> MVSKRKLSKIDAAEESSKTDLQSRCPETKRSRISDKRAPSQGGLENEGVFEELLRTSGIILKVGEGQNEIAVDQTAFQKKLRVALEKHPSYPGVVNEFISGLESHIKDRSQFKNCLLPCTPARTEGSRTLVHSYCESLIKLLLGIKILQPAVVTLLLEKIPEFFFDVVGTFGTNFPRLIVNQFKWLDGLLDSQDLVKKLMQMLSVSPVPIQHDIITSLPEILEDSQQNEVARELSCLLKQGRRLTVPILDALSRLDLDAELLAKVRQSAMTIVPSVKLEDLPVVIKFILHNVKAADAVEVISDLRKSLDLSSCVLPLQLLGSQRKLKSQAQASSSMSQVTTSQNCVKLLFDVIKLAVRFQKDVSEAWIKAIENSTSVSDHKVLDLIVLLLIHSTNSKNRKQTEKVLRSKIRLGCMPEQLMQNAFQNHSMVIKDFFPSILSLAQTFLHSAHPAVVSFGSCMYKQAFAVFDSYCQQEVVCALVTHVCSGNETELDISLDVLTDLVILHPSLLLRYATFVKTILDSMQKLNPCQIRKLFYILSTLAFSQRQEGSYIQDDMHMVIRKWLSSSVPNHKQMGIIGAVTMMGSVALKRNEADGGLLERPELSIECDGQLSTLLDLVGFCCEQTPEVLALYYDELANLIEKQKGNLDLQLLDKFGKSLVEDFPNDFVVDLSPTVDGSFLFPVKSLYNLDEDETQGAIAINLLPLVSQSEPGRVADEMSNSRKRVVSPICLSPCFRLLRLYTGEQNNGSLEEIDALLGCPLYLTDLEVEGKLDSLSKQEREFLCSLLFYALNWFREVVNAFCQQQDAEMKGKVLTRLQNITELQNVLGKCLAATPGYVPPPATFDSEAPEGVPSINAGGPVRKKNGKKRKSDSSKACSAERTQADESSDGNQPDTELSELEKSAAEKETGNPLAQLQSYRPYFRELDLEVFSVLHCGLLTKSILDTEMHTEASEVVQLGPAELCFLLDDMCWKLEHVLTPGSTRRVPFLKERGNKDVGFSHLCQRSPKEVAVCVVKLLKPLCNHMENMHNYFQTVIPNQGVVDESGLNIQEYQLMSSCYHQLLLAFRLLFAWSGFSQHENSNLLRSALQVLADRLKPGETEFLPLEELISESFQYLLNFQASIPSFQCAFILTQVLMAISEKPMTGWKREKMASLAKQFLCQSWMKPGGDREKGSHFNSALHTLLCVYLEHTDNILKAIEEISSVGVPELINSAKDGCSSTYPTLSRQTFPVFFRVMMAQLESSVKSIPAGKPSDSGEVQLEKLLKWNIAVRNFHILINLVKVFDSRPVLSICLKYGRLFVEAFLKLAMPLLDHSFKKHRDDVQSLLKTLQLSTRQLHHMCGHSKIHQDLGLTNHVPLLKKSLEQFVYRVKAMLAFNHCQEAFWVGVLKNRDLQGEEILSQASAAPEEDSAEGSEEDTEDSAAEEPDGTDSDSGGAGR;> MAQRILQLAAEGSPERLQEALQGLTEGELGDMVTRQALRGRETAALLKGIFKGSPCSQQSGVLRRLQVYKHCVSLVESGDLHVGKVSEIIGLLMLEARQLPGHALAELATLFVEVIKRGSLSNGKSLELFSTVLTALSNSKESLAYGKGELNGEEFKKQLINTLCSSKWDPQCVIHLANMFRDIPLSGEELQFVVEKVLRMFSKLDLQEIPPLVYQLLLLSAKGSKKTVLEGIISFFNQLDKRQKEEQRVPQSADLEVATVPLDQLRHVEGTVILHIVSAINLDQDIGEELIKHLKTEQQKDPGKALCPFSVSLLLSTAVKHRLQEQIFDFLKTSITRSCKDLQILQASKFLQDLCPQQYDVTAVILEVVKNSAFGWDHVTQGLVDLGFSLMESYEPKKSFGGKAAETNLGLSKMPAQQACKLGASILLETFKVHEPIRSDILEQVLNRVLTKAASPVSHFIDLLSNIVVSAPLVLQNSSSRVTETFDNLSFLPIDTVQGLLRAVQPLLKVSMSVRDSLILVLQKAIFSRQLDARKAAVAGFLLLLRNFKILGSLTSSQCSQAIGATQVQADVHACYNSAANEAFCLEILGSLRRCLSQQADVRLMLYEGFYDVLRRNSQLASSIMETLLSQIKQYYLPQQDLLPPLKLEGCIMAQGDQIFLQEPLAHLLCCIQHCLAWYKSTVHLCKGAEDEEEEEDVGFEQNFEEMLESVTRRMIKSELEDFELDKSADFSPSSGVGVKNNIYAIQVMGICEVLIEYNFKIGNFSKNKFEDVLGLFTCYNKLSEILKEKAGKNKSTLGNRIARSFLSMGFVSTLLTALFRDNAQSHEESLAVLRSSTEFMRYAVSVALQKVQQLEEMGQTDGPDGQNPEKMFQNLCKITRVLLWRYTSIPTAVEESGKKKGKSISLLCLEGLLRIFNTMQQLYAARIPQFLQALDITDGDAEEADINVTEKAAFQIRQFQRSLVNQLSSAEDDFNSKETQLLITILSTLSKLLDPGSQQFLQFLTWTVKICKENALEDLSCCKGLLTLLFSLHVLYKSPVSLLRELAQDIHACLGDIDQDVEIESRSHFAIVNVKTAAPTVCLLVLGQADKVLEEVDWLIKRLTILGSDTSEDSTQASNQTQALEKGVILQLGTLLTVFHELVQTALPAGSCVDSLLRSLSKTYAILTSLIKHYIQACRSTSNTVPGRLEKLVKLSGSHLTPQCYSFI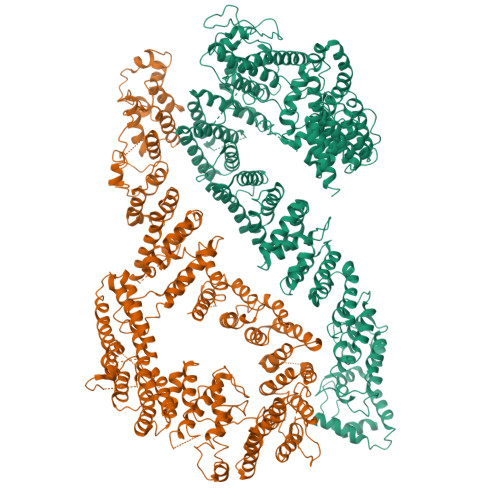TYVQNIHSESLSFAEEKKKKKKEDETAVVSTVMAKVLRDTKPIPNLIFAIEQYEKFLIHLSKKSKVNLMQYMKLSTSRDFRINASMLDSVLQEQNTEDAENEPDNNQSGTAEQPDENQEPQKKRRRKK>MSLLNNKAGVISRLADFLGFRPKTGDIDVMNRQSVGSVTISQLAKGFYEPNIESAINDVHNFSIKDVGTIITNKTGVSPEGVSQTDYWAFSGTVTDDSLPPGSPITVLVFGLPVSATTGMTAIEFVAKVRVALQEAIASFTAINSYKDHPTDGSKLEVTYLDNQKHVLSTYSTYGITISQEIISESKPGYGTWNLLG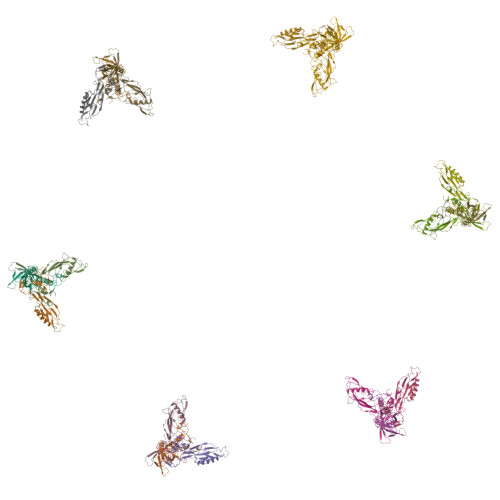AQTVTLDNQQTPTVFYHFERTA[18x]> GHMKLITAIVKPFTLDDVKTSLEDAGVLGMTVSE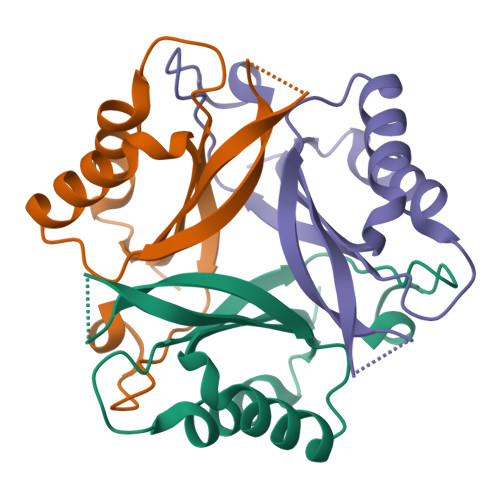IQGYGRQKGHTEVYRGAEYSVDFVPKVRIEVVVDDSIVDKVVDSIVRAARTGKIGDGKVWVSPVDTIVRVRTGERGHDAL> GPAVPRMVIEDFALNLELFRLINNARHPLLDVFFTHFAYLGSGYVLFPLLIFLFIFRKEKVKPLILAIMLETVLVISLKTFFNQPRPAILLEDVNLLFPLHWRSFPSGDTAMAFTIATVLSHGEKLHIKAILFLYAFLIGYERIYAGVHFPLDVFVGALIGIICGIISLKYSKGGVYERN

LpxE is a member of the lipid phosphatase/phosphotransferase (LPT) family, a well-distributed family of lipid-processing enzymes also known as the integral transmembrane branch of the type II phosphatidic acid phosphatase (PAP2) superfamily. This family is characterized by a conserved tripartite active site motif of KX6RP---PSGH---SRX5HX3D and activity independent of Mg2+ or other cations. Removal of the lipid A 1-phosphate by the membrane-embedded phosphatase LpxE strongly protects bacteria against host cationic peptides and the last-resort antibiotic colistin, significantly dampens the host innate immune response, and dramatically increases colonization and survival of Helicobacter pylori in the gastric mucosa. In order to gain molecular insights into the structure and function of the lipid A 1-phosphatase LpxE, we identified the previously uncharacterized gene aq_1706 from Aquifex aeolicus as the gene for the thermophilic LpxE enzyme (LpxEAA).

The selenomethionine substitution of the nonconserved I63 residue (I63M) was designed to enhance the selenium single anomalous dispersion (Se-SAD) signal for de novo phasing. The overall structure of LpxEAA contains seven α-helices, including an N-terminal amphiphilic helix lying at the periplasmic surface of the inner membrane and five tightly packed transmembrane helices (α3 to α7). Apart from α2, which originates from the periplasmic surface and penetrates halfway across the inner membrane at an ∼45° angle and immediately connects to transmembrane helix α3, the remaining helices are oriented largely in parallel or antiparallel with each other and perpendicularly to the membrane plane. Looking from the periplasmic surface, helix 5 (α5) is located at the center, which is surrounded by α2, α3, α4, α7, and α6 in a counterclockwise fashion. Fortuitously, a sulfate molecule is found in the active site, which is a structural analog of the 1-phosphate group of lipid A. The sulfate group is extensively recognized by K73 and R80 of the K73X6R80P motif and R137 of the R137X5H143X3D147 motif. The catalytically important H143 is located 3.3 Å away from the sulfur atom of the sulfate group, ready to carry out inline attack to remove the phosphate group of the lipid substrate. D147, the last residue of the R137X5H143X3D147 motif, forms a hydrogen bond with H143. The first three residues of the PSGH motif are conserved in LpxEAA, with the central serine residue (S101) serving as a helix cap to stabilize helix α5, but the histidine residue is replaced with an aspartate residue in LpxEAA. Our structural analysis of LpxEAA shows distinct features between LpxEAA and Escherichia coli PgpB (PgpBEC) enzymes but reveals a surprising structural similarity to YodM, a phosphatase of phosphatidylglycerol phosphate (PGP) in the Gram-positive bacterium Bacillus subtilis with a weak in vitro activity on undecaprenyl pyrophosphate (C55-PP).>[2x]SNLSLITKLSQEDGAILFPEIDRYSDNKQIKALTQQI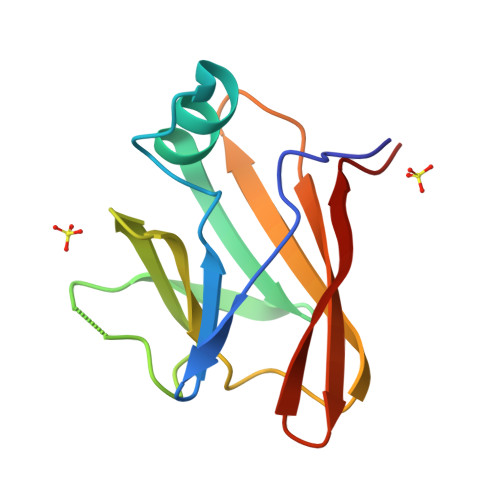TKVTVNGTVYKDLISDSVKDTNGWVSNMTGLHLGTKAFKDGENTIVISSKGFEDVTITVTKKDGQIHFVSAKQKQ>MAHHHHHHMSGMRVYLGADHAGYELKQRIIEHLKQTGHEPIDCGALRYDADDDYPAFCIAAATRTVADPGSLGIVLGGSGNGEQIAANKVPGARCALAWSVQTAALAREHNNAQLIGIGGRMHTVAEALAIVDAFV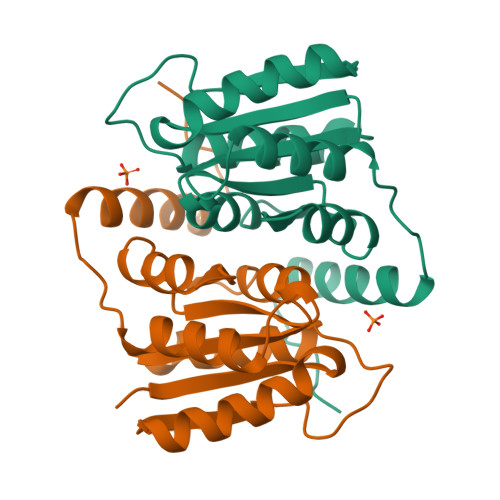TTPWSKAQRHQRRIDILAEYERTHEAPPVPGAPA[5x]>MRETDEEPEEPGRRGSFVEMVDNLRGKSGQGYYVEMTVGSPPQTLNILVDTGSSNFAVGAAPHPFLHRYYQRQLSSTYRDLRKGVYVPYTQGKWEGELGTDLVSIPHGPNVTVRANIAAITESDKFFINGSNWEGILGLAYAEIARPDDSLEPFFDSLVKQTHVPNLFSLQLCGAGFPLNQSEVLASVGGSMIIGGIDHSLYTGSLWYTPIRREWYYEVIIVRVEINGQDLKMDCKEYNYDKSIVDSGTTNLRLPKKVFEAAVKSIKAASSTEKFPDGFWLGEQLVCWQAGTTPWNIFPVISLYLMGEVTNQSFRITILPQQYLRPVEDVATSQDDCYKFAISQSSTGTVMGAVIMEGFYVVFDRARKRIGFAVSACHVHDEFRTAAVEGPFVTLDMEDCGYNIPQTDEST[2x]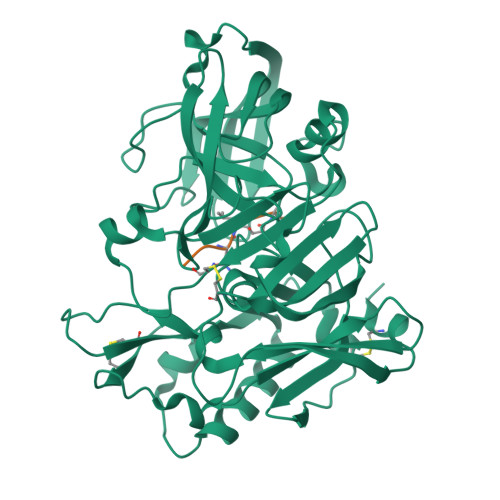;>EVNXAEF[2x]>[4x]MNTPEHMTAVVQRYVAALNAGDLDGIVALFADDATVEDGGGGEPRSGTAAIREFYANSLKLP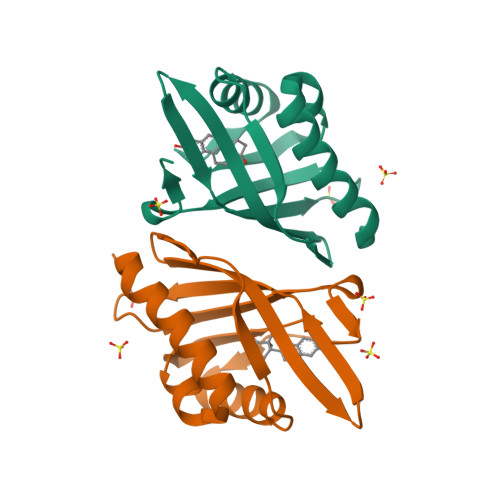LAVELTQEVRAVANEAAFAFTVSFEYQGRKTVVAPIDHFRFNGAGKVVSMRALFGEKNIHAGA> A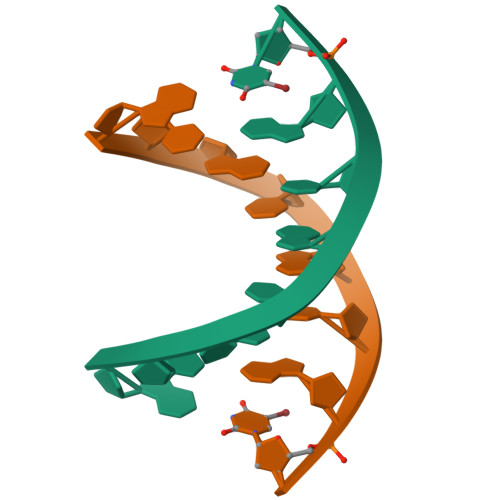CGTACGU> PIAFPFPDPPSVCELPPELAEIRDGQSVVEVKFPDGISGWMVTKHADVRKVLVDSRFSSKVMATAAAAMSETETGKLMNESLVGMDAPEHTRLRKLVTKAF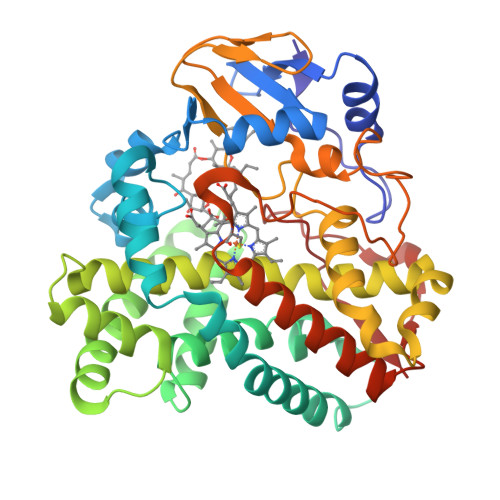TARRVETLRPRITELVGQLLDELETLPRPVDLVKNFSVPLPVRVICELLGVPAGDQDTFHAWSNALLGDWQQVVEKEAATVSLVNYFGELIAVKRENPADDLISELIAISDGDSTLTEREIIALSIGILSAGHETTANQISMFLVTLLHNPEELDKLRDNREAIPKAVDELLRFVPLTTTGGIIPRLTTAEVELSGGQVLPAGAVVLPAVATANRDPEVFEDGERLNVTRENNPHLAFGAGIHHCLGAQLARIELQEALGAILDRMPQVRLAVPESELRLKSASIIRGLESLPITW> ADVTITV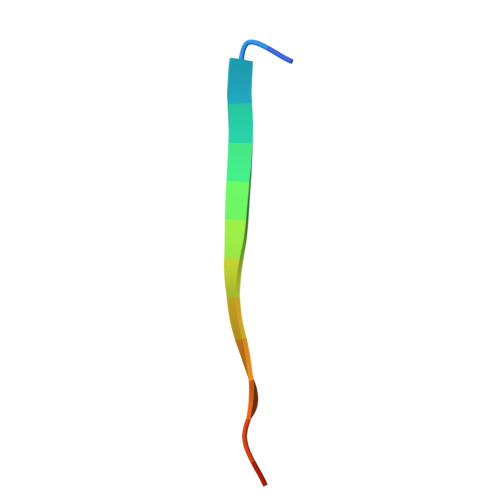NGKVVAKP>GPMGTDWPVYHRIDGP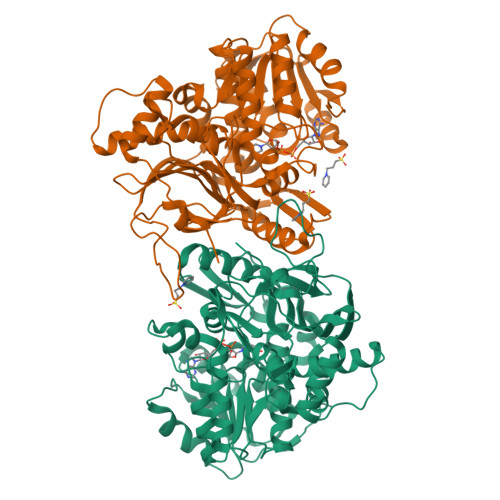IVMIGFGSIGRGTLPLIERHFAFDRSKLVVIDPSDEARKLAEARGVRFIQQAVTRDNYRELLVPLLTAGPGQGFCVNLSVDTSSLDIMELARENGALYIDTVVEPWLGFYFDPDLKPEARSNYALRETVLAARRNKPGGTTAVSCCGANPGMVSWFVKQALVNLAADLGVTGEEPTTREEWARLAMDLGVKGIHIAERDTQRASFPKPFDVFVNTFSVEGFVSEGLQPAELGWGTFERWMPDNARGHDSGCGAGIYLLQPGANTRVRSWTPTAMAQYGFLVTHNESISIADFLTVRDAAGQAVYRPTCHYAYHPCNDAVLSLHEMFGSGKRQSDWRILDETEIVDGIDELGVLLYGHGKNAYWYGSQLSIEETRRIAPDQNATGLQVSSAVLAGMVWALENPNAGIVEADDLDFRRCLEVQTPYLGPVVGVYTDWTPLAGRPGLFPEDIDTSDPWQFRNVLVRD[2x]>GSHMGNGMTKVLPGLYLGNFIDAKDLDQLGRNKITHIISIHESPQPLLQDITYLRIPVADTPEVPIKKHFKECINFIHCCRLNGGNCLVHSFAGISRSTTIVTAYVMTVTGLGWRDVLEAIKATRPIANPNP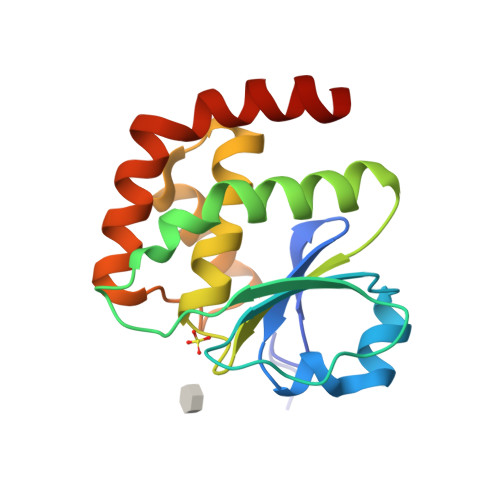GFRQQLEEFGWASSQKLRRQLEERFGES[2x]>[3x]AAPLVAETDANAKSLGYVADTTKA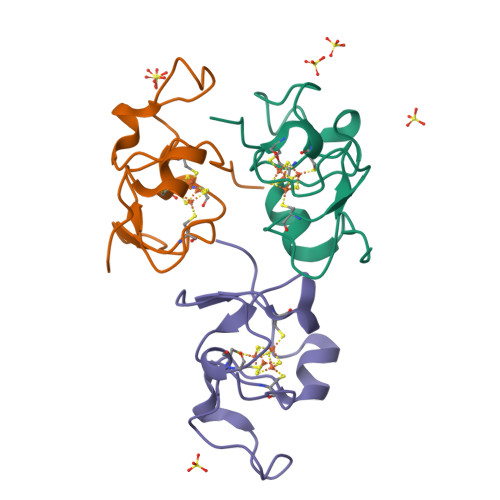DKTKYPKHTKDQSCSTCALYQGKTAPQGACPLFAGKEVVAKGWCSAWAKKA> UCCCAGUCCACCG;> CGG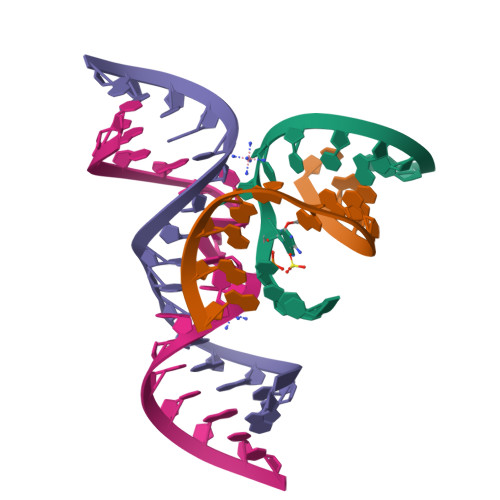UGAGAAGGG;> GGCAGAGAAACACACGA;> UCGUGGUAUAUUACCUGCC>[2x]EPKLDMNKQKISPAEVAKHNKPDDCWVVINGYVYDLTRFLPNHPGGQDVIKFNAGKDVTAIFEPLHAPNVIDKYIAPEKKLGPLQGSMPPELVCPPYAPGETKEDIARKEQLKSLLPPLDNIINLYDFEYLASQTLTKQAWAYYSSGANDEVTHRENHNAYHRIFFKPK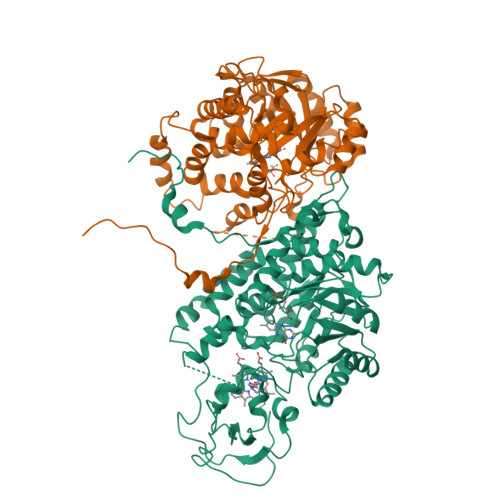ILVDVRKVDISTDMLGSHVDVPFYVSATALCKLGNPLEGEKDVARGCGQGVTKVPQMISTLASCSPEEIIEAAPSDKQIQWYQLYVNSDRKITDDLVKNVEKLGVKALFVTVDAPSLGQREKDMKLKFSNTKAGPKAMKKTNVEESQGASRALSKFIDPSLTWKDIEELKKKTKLPIVIKGVQRTEDVIKAAEIGVSGVVLSNQGGRQLDFSRAPIEVLAETMPILEQRNLKDKLEVFVDGGVRRGTDVLKALCLGAKGVGLGRPFLYANSCYGRNGVEKAIEILRDEIEMSMRLLGVTSIAELKPDLLDLSTLKARTVGVPNDVLYNEVYEGPTLTEFEDA> MNFNVSLMEKLKWKIKCIENKFLNYRLTTNETVVAETEYGKVKGVKRLTVYDDSYYSFEGIPYAQPPVGELRFKAPQRPTPWDGVRDCCNHKDKSVQVDFITGKVCGSEDCLYLSVYTNNLNPETKRPVLVYIHGGGFIIGENHRDMYGPDYFIKKDVVLINIQYRLGALGFLSLNSEDLNVPGNAGLKDQVMALRWIKNNCANFGGNPDNITVFGESAGAASTHYMMLTEQTRGLFHRGILMSGNAICPWANTQCQHRAFTLAKLAG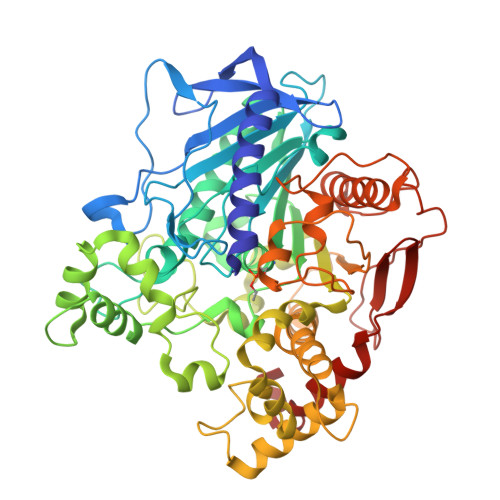YKGEDNDKDVLEFLMKAKPQDLIKLEEKVLTLEERTNKVMFPFGPTVEPYQTADCVLPKHPREMVKTAWGNSIPTMMGNTSYEGLFFTSILKQMPLLVKELETCVNFVPSELADAERTAPETLEMGAKIKKAHVTGETPTADNFMDLCSHFYFWFPMHRLLQLRFNHTSGTPVYLYRFDFDSEDLINPYRIMRSGRGVKGVSHTDELTYFFWNQLAKRMPKESREYKTIERMTGIWTQFATTGNPYSNEIEGMENVSWDPIEKSDEVYKCLNISDELKMIDVPEMGKIKQWESMFEKHRDLF> PDHELVVCGAPDAAALTGLLTRVRAAATALSRPELTDLAAGLAAAHRGDVPARFAAAVRDADGLVAALDRALGHLAEGGRRLLDAGRGLFLVVGG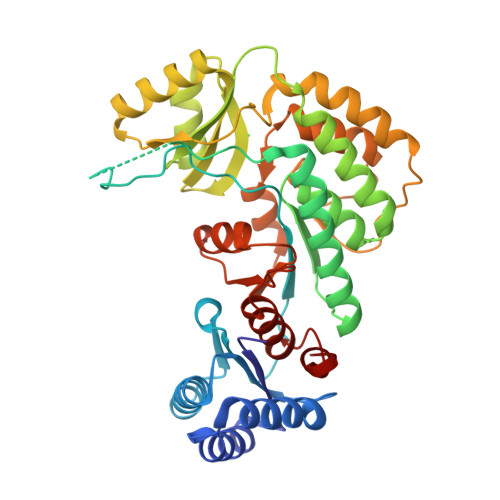PLRVGLLFPGQAAPVHADRGALGHLLGDADAGTGSDPDSGVKPAEPVDTAVAQPAIIADSLAGIRWLDRLGARPVGALGHSLGELAALSWAGALDADDTLALARARGEAMSAATEAPSGMLSLRADLAAARELAAGTGAVVAVDNGERHVVVAGTRPELDRVAEAARHAGIEATPLAVSHAFHSPLMAPAAEALRRAAGRLPWRRPERPVASTVTGAWWADEDPVEVLVRQLTGPVRFREALGLLDADLLVEVGPGRMLSALAEAAGRTAVSLDAGAASAAGMAAGTAALFAAGAVDDATPFFAGR>MQVIPACNSAAIRSLCPTPESFRNMGWLSVSDAVYSEFIGELATRASNRNYSNEFGLMQPIQEFKAFIESDPVVHQEFIDMFEGIQDSPRNYQELCNMFNDIFRKAPVYGDLGPPVYMIMAKLMNTRAGFSAFTRQRLNLHFKKLFDTWGLFLSSKDSRNVLVADQFDDRHCGWLNERALSAMVKHYNGRAFDEVFLCDKNAPYYGFNSYDDFFNRRFRNRDIDRPVVGGVNNTTLISAACESLSYNVSYDVQSLDTLVFKGETYSLKHLLNNDPFTPQFEHGSILQGFLNVTAYHRWHAPVNGTIVKIINVPGTYFAQAPSTIGDPIPDNDYDPPPYLKSLVYFSNIAARQIMFIEADNKEIGLIFLVFIGMTEISTCEATVSEGQHVNRGDDLGMFHF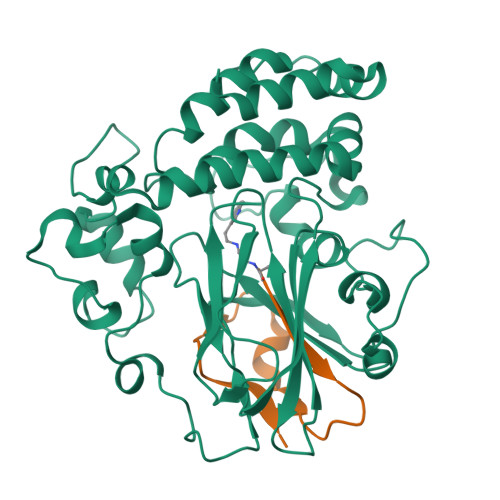GG[6x];>[6x]SFALGLRKDCRAEIVEKFTEPGTVIRINEVVAALKA> MIRLYPEQLRAQLNEGLRAAYLLLGNDPLLLQESQDAVRQVAAAQGFEEHHTFSIDPNTDWNAIFSLCQAMSLFASRQTLLLLLPENGPNAAINEQLLTLTGLLHDDLLLIVRGNKLSKAQENAAWFTALANRSVQVTCQTPEQAQLPRWVAARAKQLNLELDDAANQVLCYCYEGNLLALAQALERLSLLWPDGKLTLPRVEQAVNDAAHFTPFHWVDALLMGKSKRALHILQQLRLEGSEPVILLRTLQRELLLLVNLKRQSAHTPLRALFDKHRVWQNRRGMMGEALNRLSQTQLRQAVQLLTRTELTLKQDYGQSVWAELEGLSLLLCH;>GPHMSYQVLARKWRPQTFADVVGQEHVLTALANGLSLGRIHHAYLFSGTRGVGKTSIARLLAKGLNCETGITATPCGVCDNCREIEQGRFVDLIEIDAASRTKVEDTRDLLDNVQYAPARGRFKVYLIDEVHMLSRHSFNALLKTLEEPPEHVKFLLATTDPQKLPVTILSRCLQFHLKALDVEQIRHQLEHILNEEHIAHEPRALQLLARAAEGSLRDALSLTDQAIASGDGQVSTQAVSAMLGTLDDDQALSLVEAMVEANGERVMALINEAAARGIEWEALLVEMLGLLHRIAMVQLSPAALGNDMAAIELRMRELARTIPPTDIQLYYQTLLIGRKELPYAPDRRMGVEMTLLRALAFHPRMPLPEPEVPRQ[3x];> GPHMRWYPWLRPDFEKLVASYQAGRGHHALLIQALPGMGDDALIYALSRYLLCQQPQGHKSCGHCRGCQLMQAGTHPDYYTLAPEKGKNTLGVDAVREVTEKLNEHARLGGAKVVWVTDAALLTDAAANALLKTLEEPPAETWFFLATREPERLLATLRSRCRLHYLAPPPEQYAVTWLSREVTMSQDALLAALRLSAGSPGAALALFQGDNWQARETLCQALAYSVPSGDWYSLLAALNHEQAPARLHWLATLLMDALKRHHGAAQVTNVDVPGLVAELANHLSPSRLQAILGDVCHIREQLMSVTGINRELLITDLLLRIEHYLQPGVVLPVPHL;>[2x]GPHMKFTVEREHLLKPLQQVSGPLGGRPTLPILGNLLLQVADGTLSLTGTDLEMEMVARVALVQPHEPGATTVPARKFFDICRGLPEGAEIAVQLEGERMLVRSGRSRFSLSTLPAADFPNLDDWQSEVEFTLPQATMKRLIEATQFSMAHQDVRYYLNGMLFETEGEELRTVATDGHRLAVCSMPIGQSLPSHSVIVPRKGVIELMRMLDGGDNPLRVQIGSNNIRAHVGDFIFTSKLVDGRFPDYRRVLPKNPDKHLEAGCDLLKQAFARAAILSNEKFRGVRLYVSENQLKITANNPEQEEAEEILDVTYSGAEMEIGFNVSYVLDVLNALKCENVRMMLTDSVSSVQIEDAASQSAAYVVMPMRL

Clamp loaders are pentameric ATPases that place circular sliding clamps onto DNA, where they function in DNA replication and genome integrity. Because the sliding clamp is a closed ring in solution, it needs to be opened and placed onto DNA by a separate ATPase complex called the clamp loader. All clamp loaders are pentameric ATPases of the AAA + family (ATPases associated with various cellular activities). Here we describe a series of structures of the E. coli clamp loader in the process of placing the clamp onto a p/t-junction.

In micrographs of the sample containing ADP·BeFx, we observe two different conformations of the clamp loader/sliding clamp complex, both with the clamp open. However, the degree of opening is drastically different between these two states. In the second state, the sliding clamp is opened into a wide, planar conformation (overall resolution = 3.0 Å). Therefore, we designate these two states as the Semi-Open and the Fully-Open states, respectively. As in the Semi-Open state, all five subunits of the clamp loader also make contact with the sliding clamp in the Fully-Open state. The primary conformational change between these two states is a dramatic increase in interfacial contacts between the B and C subunits. This is accomplished by a single pivoting motion at a point between the B and C subunits. Because the B and C subunits are contacting the sliding clamp, this pivoting motion imparts an equivalent pivoting motion within subunit I of the sliding clamp, resulting in the wide planar opening. In both the Semi- and Fully-Open states, there is no significant density for Domain I of the second subunit of the ß-clamp, which is at the site of the ring opening. In the Fully-Open state, the arginine finger of the C subunit contacts the B subunit’s ATP.> MDSSTWSPKTTAVTRPVETHELIRNAADISIIVIYFVVVMAVGLWAMFSTNRGTVGGFFLAGRSMVWWPIGASLFASNIGSGHFVGLAGTGAASGIAIGGFEWNALVLVVVLGWLFVPIYIKAGVVTMPEYLRKRFGGQRIQVYLSLLSLLLYIFTKISADIFSGAIFINLALGLNLYLAIFLLLAITALYTITGGLAAVIYTDTLQTVIMLVGSLILTGFAFHEVGGYDAFMEKYMKAIPTIVSDGNTTFQEKCYTPRADSFHIFRDPLTGDLPWPGFIFGMSILTLWYWCTDQVIVQRCLSAKNMSHVKGGCILCGYLKLMPMFIMVMPGMISRILYTEKIACVVPSECEKYCGTKVGCTNIAYPTLVVELMPNGLRGLMLSVMLASLMSSLTSIFNSASTLFTMDIYAKVRKRASEKELMIAGRLFILVLIGISIAWVPIVQSAQSGQLFDYIQSITSYLGPPIAAVFLLAIFWKRVNEPGAFWGLILGLLIGISRMITEFAYGTGSCMEPSNCPTIICGVHYLYFAIILFAISFITIVVISLLTKPIPDVHLYRLCWSLRNSKEERIDLDAEEENIQEGPKETIEIETQVPEKKKGIFRRAYDLFCGLEQHGAPKMTEEEEKAMKMKMTDTSEKPLWRTVLNVNGIILVTVAVFCHAYFA;> MSALSLLILGLLTAVPPASCQQGLGNLQPWMQGLIAVAVFLVLVAIAFAVNHFWCQEEPEPAHMILTVGNKADGVLVGTDGRYSSMAASFRSSEHENAYENVPEEEGKVRSTPM

The uptake of glucose against its concentration gradient is mediated by the sodium-dependent glucose cotransporters (SGLT). These transporters utilize the electrochemical gradient to drive the uphill transport of glucose and play essential roles in human health. SGLT1 (SLC5A1) and SGLT2 (SLC5A2) are two important subtypes of this family, and their physiological functions are well-documented. Pioneering structural work on the bacterial homolog vSGLT from Vibrio parahaemolyticus revealed that SGLT proteins have 14 transmembrane helices, which assemble into a LeuT-like fold.

We adopted the “three-joint-tethering” strategy to generate the fully functional hSGLT1GFP-MAP17nb protein for structural studies. It was reported that replacing the equatorial hydroxyl group at the 4-position of glucose with a fluorine atom yielded a glucose analogue, 4-deoxy-4-fluoro-d-glucose (4D4FDG), with an enhanced affinity for SGLT1 (K0.5 is 0.07 mM) compared with glucose (K0.5 is 0.5 mM). Therefore, to obtain the structure of hSGLT1 in the substrate-bound state, we supplemented the hSGLT1GFP-MAP17nb protein with 4D4FDG throughout the purification, the nanodisc reconstitution, and the cryo-EM sample preparation. Single particle analysis yielded a reconstruction of the hSGLT1-4D4FDG complex at 3.26 Å resolution. A ligand density was found at the sugar-binding pocket of hSGLT1. The surface representation of the hSGLT1-4D4FDG complex shows the substrate-binding site is occluded to both the extracellular and intracellular solvent. 4D4FDG is caged inside a cavity surrounded by TM1, TM2, TM3, TM6, TM7, and TM10. Above the sugar-binding site, I98 and F101 on TM2, M283 on TM6, and F453 and Q457 on TM10 block the substrate entry pathway from the extracellular solution. Below the sugar-binding site, N78 on TM1, Y290 and W291 on TM6 form the first layer of insulation. S77 on TM1, V296 on TM6, and S396 on TM8 form the second layer of insulation. In the extracellular vestibule, F453 moves 3.8 Å inwardly due to the rotation of TM10a and forms hydrophobic interactions with I98 and F101 on TM2 to close the extracellular gate.>[2x]GHMQEKPPKELVNEWSL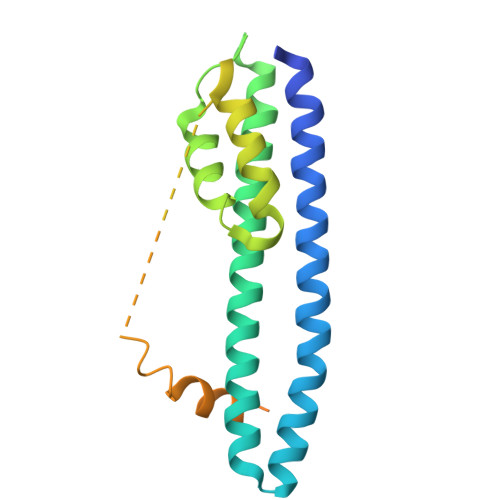KIRKEMRVVDRQIRDIQREEEKVKRSVKDAAKKGQKDVCIVLAKEMIRSRKAVSKLYASKAHMNSVLMGMKNQLAVLRVAGSLQKSTEVMKAMQSLVKIPEIQATMRELSKEMMKAGIIEEMLEDTFESMDDQEEMEEEAEMEIDRILFEITAGALGKAPSKVTDALPEPEPPGAMAASEDEEEEEEALEAMQSRLATLRS>[2x]MLRLSAPGQLDDDLCLLGDVQVPVFLLRLGEASWALVEGGISRDAELVWADLCRWVADPSQVHYWLITHKHYDHCGLLPYLCPRLPNVQVLASERTCQAWKSESAVRVVERLNRQLLRAEQRLPEACAWDALPVRAVADGEWLELGPRHRLQVIEAHGHSDDHVVFYDVRRRRLFCGDALGEFDEAEGVWRPLVFDDMEAYLESLERLQRLPTLLQLIPGHGGLLRGRLAADGAESAYTECLRLCRRLLWRQSMGESLDELSEELHRAWGGQSVDFLPGELHLGSMRRMLEILSRQALPLD;>MRNDGGFLLWWDGLRSEMQPIHDSQGVFAVL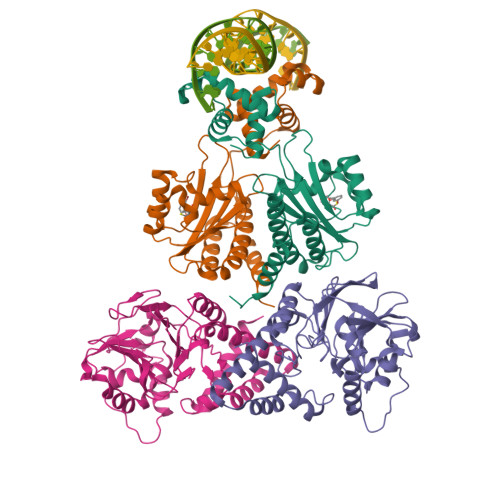EKEVRRLGFDYYAYGVRHTIPFTRPKTEVHGTYPKAWLERYQMQNYGAVDPAILNGLRSSEMVVWSDSLFDQSRMLWNEARDWGLCVGATLPIRAPNNLLSVLSVARDQQNISSFEREEIRLRLRCMIELLTQKLTDLEHPMLMSNPVCLSHREREILQWTADGKSSGEIAIILSISESTVNFHHKNIQKKFDAPNKTLAAAYAAALGLI[2x]>GSKKHSVLHLVPVNITSKADSDVTEVMWQPVLRRGRGLEAQGDIVRVWDTGIYLLYSQVLFHDVTFTMGQVVSREGQGRRETLFRCIRSMPSDPDRAYNSCYSAGVFHLHQGDIITVKIPRANAKLSLSPH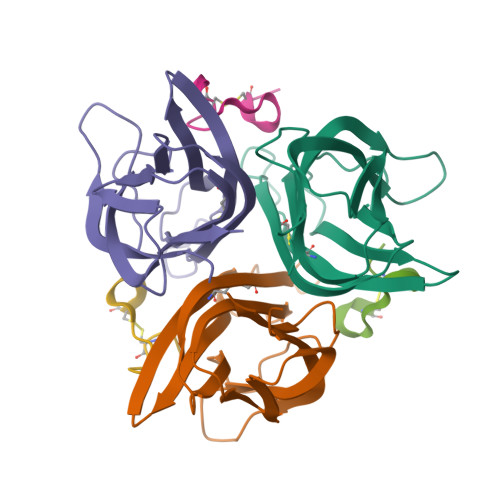GTFLGFVKL[3x];>SGWCDPRWYDPFMCEH[3x]> MAMSNMTYNNVFDHAYEMLKENIRYDD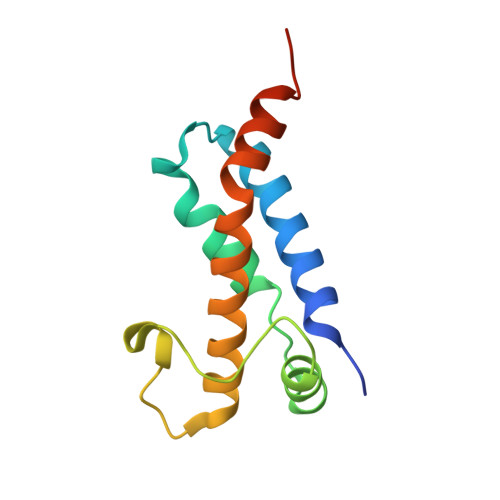IRDTDDLHDAIHMAADNAVPHYYADIFSVMASEGIDLEFEDSGLMPDTKDVIRILQARIYEQLTIDLWEDAEDLLNEYLEEVEEYEEDEE>[2x]MADYKDDDDKSGRMPHFTVTKVEDPEEGAAASI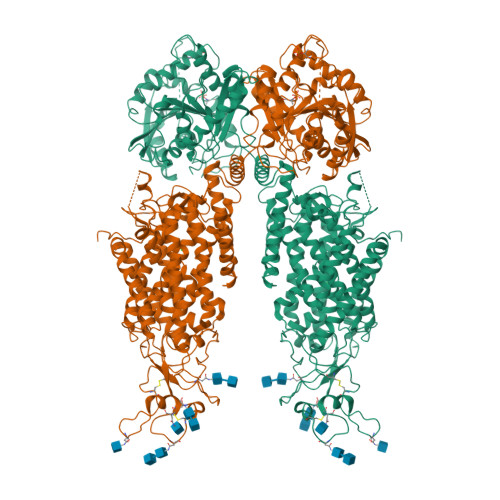SQEPSLADIKARIQDSDEPDLSQNSITGEHSQLLDDGHKKARNAYLNNSNYEEGDEYFDKNLALFEEEMDTRPKVSSLLNRMANYTNLTQGAKEHEEAENITEGKKKPTKTPQMGTFMGVYLPCLQNIFGVILFLRLTWVVGTAGVLQAFAIVLICCCCTMLTAISMSAIATNGVVPAGGSYFMISRALGPEFGGAVGLCFYLGTTFAAAMYILGAIEIFLVYIVPRAAIFHSDDALKESAAMLNNMRVYGTAFLVLMVLVVFIGVRYVNKFASLFLACVIVSILAIYAGAIKSSFAPPHFPVCMLGNRTLSSRHIDVCSKTKEINNMTVPSKLWGFFCNSSQFFNATCDEYFVHNNVTSIQGIPGLASGIITENLWSNYLPKGEIIEKPSAKSSDVLGSLNHEYVLVDITTSFTLLVGIFFPSVTGIMAGSNRSGDLKDAQKSIPIGTILAILTTSFVYLSNVVLFGACIEGVVLRDKFGDAVKGNLVVGTLSWPSPWVIVIGSFFSTCGAGLQSLTGAPRLLQAIAKDNIIPFLRVFGHSKANGEPTWALLLTAAIAELGILIASLDLVAPILSMFFLMCYLFVNLACALQTLLRTPNWRPRFRYYHWALSFMGMSICLALMFISSWYYAIVAMVIAGMIYKYIEYQGAEKEWGDGIRGLSLSAARFALLRLEEGPPHTKNWRPQLLVLLKLDEDLHVKHPRLLTFASQLKAGKGLTIVGSVIVGNFLENYGEALAAEQTIKHLMEAEKVKGFCQLVVAAKLREGISHLIQSCGLGGMKHNTVVMGWPNGWRQSEDARAWKTFIGTVRVTTAAHLALLVAKNISFFPSNVEQFSEGNIDVWWIVHDGGMLMLLPFLLKQHKVWRKCSIRIFTVAQLEDNSIQMKKDLATFLYHLRIEAEVEVVEMHDSDISAYTYERTLMMEQRSQMLRHMRLSKTERDREAQLVKDRNSMLRLTSIGSDEDEETETYQEKVHMTWTKDKYMASRGQKAKSMEGFQDLLNMRPDQSNVRRMHTAVKLNEVIVNKSHEAKLVLLNMPGPPRNPEGDENYMEFLEVLTEGLERVLLVRGGGSEVITIYS Here we have determined by cryo-electron microscopy (cryo-EM) structures of the head and tail components of YSD1, a phage infecting Salmonella Typhi. We investigated the structure of the recently characterised phage YSD1 as an example of flagellotropic χ-like phages and more generally phages with long, non-contractile tails. Samples of YSD1 imaged by EM showed characteristic features of siphoviruses: an icosahedral capsid and a flexible tail tube of ~220 nm in length. Cryo-EM analysis of YSD1 allowed structure determination of the head and tail components at resolutions of 3.8 Å and 3.5 Å, respectively, and the generation of de novo models for the major capsid (YSD1_17), auxiliary protein (YSD1_16) and tail-tube protein (YSD1_22).

To investigate the assembly of the major capsid component, we determined the structures of the major capsid protein both within the assembled head by cryo-EM and in its soluble form by X-ray crystallography of the recombinant protein (resolution: 2.6 Å). Comparison of the two structures revealed major rearrangements correlating with the transition from a soluble, monomeric form to an assembled capsid. These rearrangements are unlikely to be caused by crystal packing since the same compact conformations are seen for both of the independent molecules in the asymmetric unit of the crystal despite completely different environments. Taking the compact crystal structure as a reference, these rearrangements can be described as the stretch of the N-terminal arm and E-loop in opposite directions with regard to the central P-domain. In these conformations, the two structural elements form an inter-molecular beta-sheet with their counterparts of the neigboring subunits within a capsomer, which results in a circular strand exchange. In addition to interlocking the capsomer, these interactions allow for quasi-equivalent interactions modulated by varying bending angles of the N-terminal arm and E-loop. These quasi-equivalent interactions observed in the asymmetric unit of the capsid ultimately allow the formation of pentamers and hexamers with different curvatures, which are required to assemble the large T7 icosahedral shell.

>MAGLYTTYQLLEVQRKLKTLPAFFLQWFPRQINFQEDMIAFDKVIQDVTRVAPFVAPNVQGRVIKESGYNTKTFKPAYVKPKHVIDPNMIIPRQPGEALGTGTLSIAQRRDRVIAYLLMKHRAMHENTWEWMAAQAAQYGYVDVQGQDYPLVRVDFGRDAALTMTTDWTAAGVTLMDMIADLRDGQRLVSDKSMSGTVIRDYVFGGDAWDQFVKVGGKELWGKDGLMDSTIRGSETNVTRLWDDVEGVQYMGELVGANGAGRMRIWVNTQKYRDQNDQEQFLMKQKAVMGISSAIEGVRCFGAILDKGAGYQALDYFPKMWDQEDPSVEYLMSQGAPLMVPADPNASFLLTVMS[2x]> MSKPQPIAAANWKSGSPDSL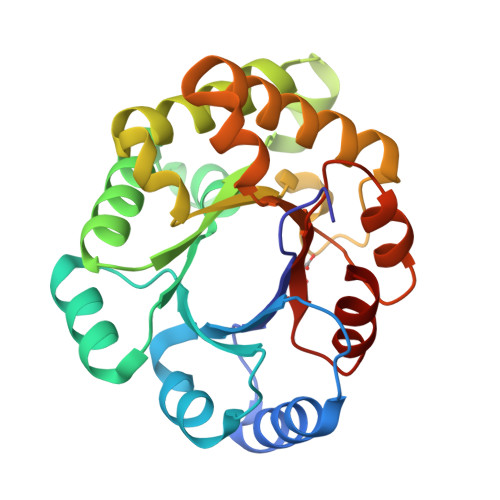SELIDLFNSTSINHDVQCVVASTFVHLAMTKERLSHPKFVIAALNAGNADALASLKDFGVNWIVLGHSERRWYYGETNEIVADKVAAAVASGFMVIACIGETLQERESGRTAVVVLTQIAAIAKKLKKADWAKVVIAYEPVWAIGTGKVATPQQAQEAHALIRSWVSSKIGADVAGELRILYGGSVNGKNARTLYQQRDVNGFLAGLKPEFVDIIKATQ> GPGHAGIFTFEEPVTHVSESIGIMEVKVLRTSGARGNVIVPYKTIEGTARGGGEDFEDTCGELEFQNDEIVKTISVKVIDDEEYEKNKTFFLEIGEPRLVEMSEKKALLLNELGGFTITGK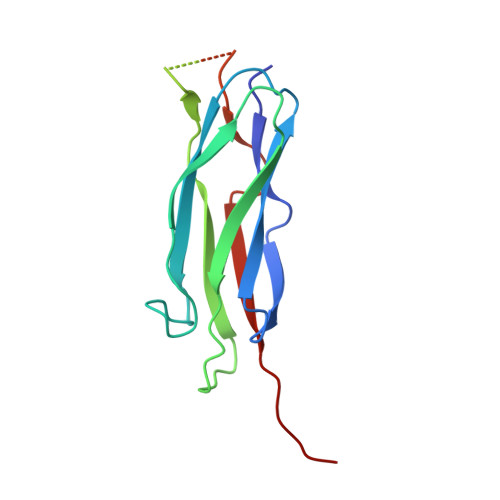YLYGQPVFRKVHAREHPIPSTVITIAEEYDDKQPLTSKEEEERRIAEMGRPILGEHTKLEVIIEESYEFKS> GPNRIKLVPIAPSRGIIYDRNGIPLALNRTIYQIEMMPEKVDNVQQTLDALRSVVDLTDDDIAAFRKERARSHRFTSIPVKTNLTEVQVARFAVNQYRFPGVEVKGYKRRYYPYGSALTHVIGYVSKINDKDVERLNNDGKLANYAATHDIGKLGIERYYEDVLHGQTGYEEVEVNNRGRVIRQLKEVPPQAGHDIYLTLDLKLQQYIETLLAGSRAAVVVTDPRTGGVLALVSTPSYDPNLFVDGISSKDYSALLNDPNTPLVNRATQGVYPPASTVKPYVAVSALSAGVITRNTTLFDPGWWQLPGSEKRYRDWKKWGHGRLNVTRSLEESADTFFYQVAYDMGIDRLSEWMGKFGYGHYTGIDLAEERSGNMPTREWKQKRFKKPWYQGDTIPVGIGQGYWTATPIQMSKALMILINDGIV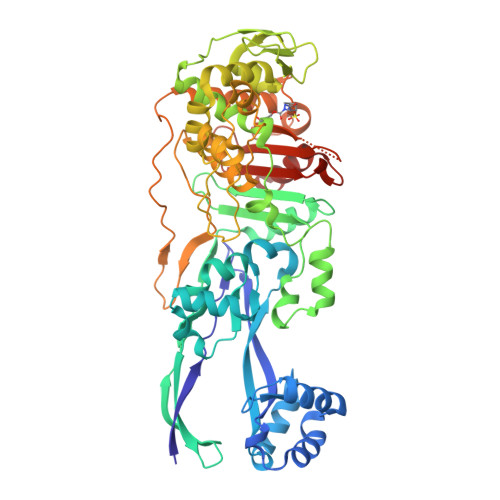KVPHLLMSTAEDGKQVPWVQPHEPPVGDIHSGYWELAKDGMYGVANRPNGTAHKYFASAPYKIAAKSGTAQVFGLKANETYNAHKIAERLRDHKLMTAFAPYNNPQVAVAMILENGGAGPAVGTLMRQILDHIMLGD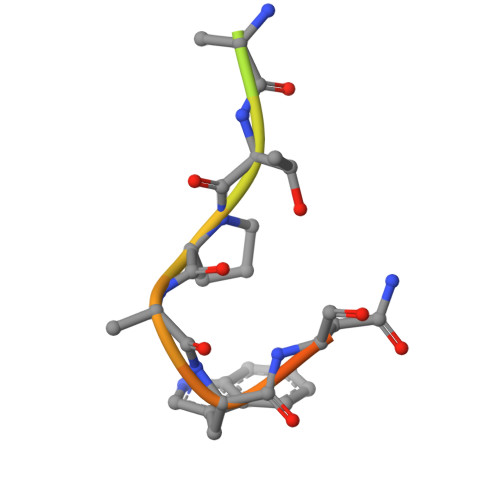> TPAWNSGSRTPAWNSGSK> NADDQLKQLSALEGANGYVIFNESGIPLKRHEKSISHEKAVHIAALVSDLWNVSKKVIQRDLKTPENDIEVIRLRTKHSYEYIITQ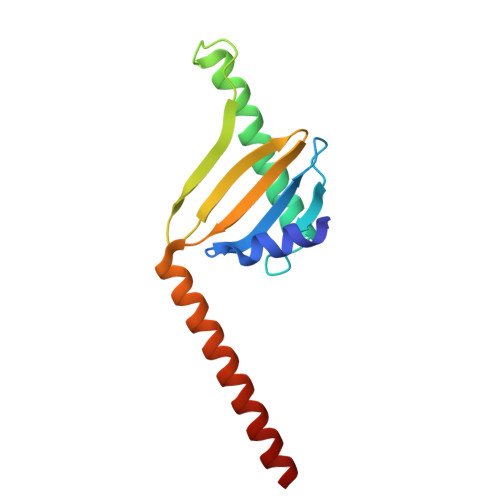SGDFTMLAIQLCGKAIEEAKKAAAAAAAAAVVQEENKEKEKK> DKVYE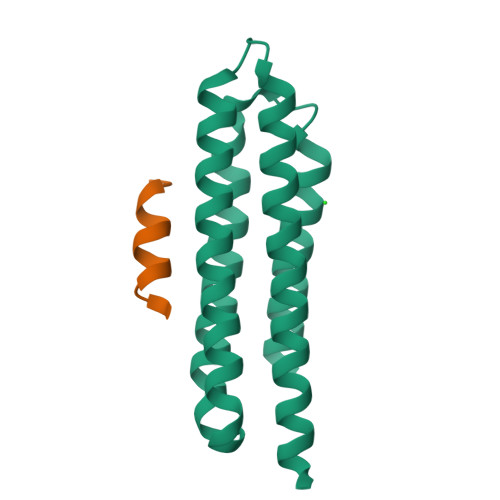NVTGLVKAVIEMSSKIQPAPPEEYVPMVKEVGLALRTLLATVDETIPLLPASTHREIEMAQKLLNSDLGELINKMKLAQQYVMTSLQQEYKKQMLTAAHALAVDAKNLLDVIDQARLKMLG As the most abundant viral protein encoded by the M gene segment, matrix protein 1 (M1) forms a shell underneath a host cell-derived lipid biolayer to connect the vRNPs with the viral envelope in mature virions. The full-length M1 protein includes 252 amino acids consisting of a highly organized N-terminal domain and a flexible but less ordered C-terminal domain that are linked by a protease-sensitive loop. So far, only the N-terminal domain of M1 has been structurally resolved at an atomic level, showing that at neutral pH the physiological monomers have a high tendency to oligomerize via a so-called ‘face-to-back’ arrangement, whereas at acidic pH the N-terminal domain exists as a dimeric structure in a so-called ‘face-to-face’ arrangement.

In sharp contrast to M(NLS-88R), both M(NLS-88E) neutral and acidic structures are in a face-to-face-oriented dimeric mode and lack pH-dependent conformational switches. As for M(NLS-88E)-acidic structure, it contains two face-to-face-arranged dimers. On the other side, M(NLS-88E)-acidic has monomers A and B associate in a face-to-face arrangement to form dimer 1, and has molecule C similarly associated with its dyad equivalent to form dimer 2. All three M(NLS-88E)-acidic monomers superposed on each other with a r.m.s.d. of ~0.5 Å. However, least-squares superposition of the two M(NLS-88E)-acidic independent dimers 1 and 2 resulted in a very large r.m.s.d. of 1.2 Å, indicating that the two dimers of M(NLS-88E)-acidic show significantly different dimer arrangements. Dimer 1 of M(NLS-88E)-acidic is more like M(NLS-88E)-neutral dimer (r.m.s.d. of ~0.6 Å screw rotation angle of ~8°), but not its dimer 2 (r.m.s.d. of ~0.6 Å screw rotation angle of ~15°). However, dimer 1 of M(NLS-88E)-acidic is more like M(NLS-88E)-neutral that owns a strong bifurcated hydrogen-bond interaction between Tyr100 and Glu88 because of the G88E mutation that makes it more difficult to dissemble M(NLS-88E) M1 in acidic conditions than M(NLS-88R) M1. Dimer 2 of M(NLS-88E)-acidic is significantly different from all other obtained dimeric structures by showing neither apparent contact between Asn85 and Arg134 nor apparent inter-subunit interaction involving Glu88. Dimer 2 of M(NLS-88E)-acidic likely represents an intermediate conformation due to incomplete transition after the pH drops.

>[3x]MHHHHHHSLLTEVETYVLSIVPSGPLKAEIAQRLEDVFAGKNTDLEVLMEWLKTRPILSPLTKGILGFVFTLTVPSERGLQRRRFVQNALNGNEDPNNMDKAVKLYSKLKSEITFHGAKEIALSYSAGALASCMGLIYNRMGAVTTEVAFGLVCATCEQIADSQHRSHRQM>SNSRAADQLELDGLPGTPPDFYRERQRSRVERYQSPAGAPLQCSVQVQTTQEHPLWTSHVWSGARALADTLCWQPELIAGKTVCELGAGAGLVSIVAFLAGADQVVATDYPDPEILNSLESNIREHTA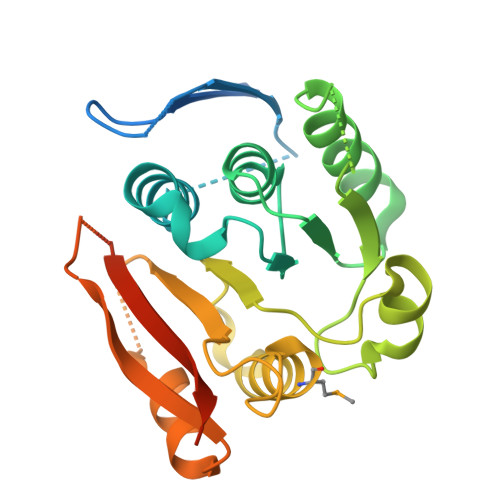NSCSSETVKRASPKVVPYRWGDSPDSLQRCTGLQRFQVVLLADLLSFHQAHDALLRSVKMLLALPANDPTAVALVTFTHHRPHLAERDLAFFRLVNADGALIAEPWLSPLQMDPMFPDDPGDVCIRGQVHRWRLRWRSAASASANIPAHARNE[2x]>GPGYQDPNSVMTTKGHIYVIDDDAAMRDSLNFLLDSAGFGVTLFDDAQAFLDALPGLSFGCVVSDVRMPGLDGIELLKRMKAQQSPFPILIMTGHGDVPLAVEAMKLGAVD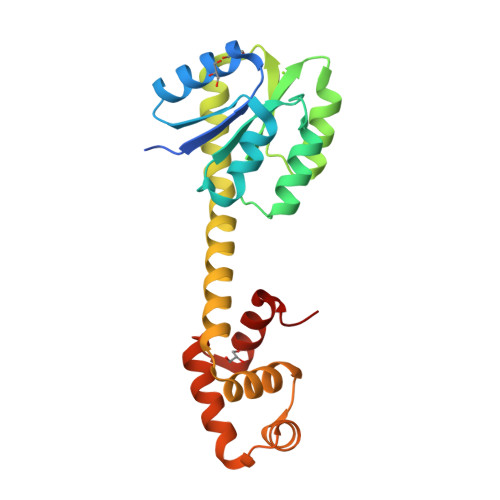FLEKPFEDDRLTAMIESAIRQAEPAAKSEAVAQDIAARVASLSPRERQVMEGLIAGLSNKLIAREYDISPRTIEVYRANVMTKMQANSLSELVRLAMRAGMLND[5x]> NEYAPLRLHVPEPTGRPGCQTDFSYL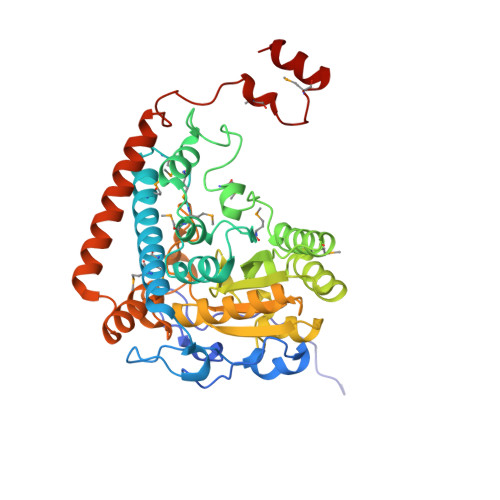RLNDAGQARKPPVDVDAADTADLSYSLVRVLDEQGDAQGPWAEDIDPQILRQGMRAMLKTRIFDSRMVVAQRQKKMSFYMQSLGEEAIGSGQALALNRTDMCFPTYRQQSILMARDVSLVEMICQLLSNERDPLKGRQLPIMYSVREAGFFTISGNLATQFVQAVGWAMASAIKGDTKIASAWIGDGATAESDFHTALTFAHVYRAPVILNVVNNQWAISTFQAIAGGESTTFAGRGVGCGIASLRVDGNDFVAVYAASRWAAERARRGLGPSLIEWVTYRAGPHSTSDDPSKYRPADDWSHFPLGDPIARLKQHLIKIGHWSEEEHQATTAEFEAAVIAAQKEAEQYGTLANGHIPSAASMFEDVYKEMPDHLRRQRQEL> MESGIDLQGQFISALQSLGLSHDLAKLLWLPLPMLMMLIVATVGVLVAVWLERKISAAVQQRIGPEYIGPLGILAPLADGLKLIFKEDVLPANSDRWLFTLGPAVVVIPVFLSYIIVPFGQNLLISNLAMGVFLWIALSSIAPIGLLMAGYASNNKYSLLGGLRAAAQSISYEIPLALAVLAVAMMSNGLGTVEIVEQQSQYGILSWNVWRQPIGFLVFWIAALAECERLPFDLPEAEEELVAGYQTEYAGMKFALFYLGAYVNLVLSALLVSVLYFGGWSFPIPLETIANLLGVSETNPFLQIAFAVLGITMTLIKAYFFVFLAILLRWTVPRVRIDQLLDLGWKFLLPVGLVNLLLTAGLKLAFPVAFGG;> MDLVTLAGQLNAGTILPETILIVTLLVVLLADLIQGRQADRWTPYFAIVGLGGAIATMIPLWTQPATISFFGSFISDHLSLFFRGLIALSALGTILMSIRYVEQTGSSLGEFMTILLTATVGGMFIAGAQELVFIFVALETLSIASYLLTGYTKRDSRSNEAALKYLLIGAASSAIFLYGSSLLYGLSGGHTQLPAIAQALSSESLGLVVALVFVIAGISFKISAVPFHQWTPDVYEGAPTPVVAFLSVGSKAAGFALAIRFLTLAFPSVTDQWQLIFTVLAILSMILGNVVALAQTSMKRMLAYSSIGQAGFVMIGFVVGTEAGYASMLFYLLVYLFMNLGAFTCVILFSLRTGTDQISEYAGLYQKDPLLTLGLSLCLLSLGGIPPLAGFFGKIYLFWAGWQAGAYGLVLLGLLTSVISIYYYIRVVKMMVVKEPQEMSEAVRNYPEVSWSSFGLRPLQVGLVMTVIATSLAGILANPLFNLVNTAVWDVPQLANQPTVMEVAYQALSPAGKS;> MVAIPRLRDTATVFVLSGYEYFLGFLIICSLVPVLALAASALLRPKSGRMIRLTTYESGMEPIGGAWIQFNVRYYMFALVFVIFDVETVFLYPWAVAFHQLGLLAFIEALIFIAILVVALVYAWRKRALEWS;> MSTFPWLTTIILFPIVAALAIPFIPDPTGKGRPIRWYALAVGLIDFALIVYAFTNFYDLNTPGMQLWESYDWIPEIGLRWSVGADGLSMPLILLTGFITTLAILAAWPVTLKPRLFYFLMLAMYGGQIAVFAVQDMLVFFLAWELELIPVYLLLAIWGGHKRQYAATKFILYTAGSSLFILVAGLAMAFYGDTVSFDMQTLAAKDYALGFQLLVYAGFLVAYGVKLPIVPLHTWLPDAHGEATAPVHMLLAGILLKMGGYALIRMNVDMLPAAHAKFAPVLVILGVVNIIYAALTSYAQRNLKRKIAYSSISHIGFVLIGIASFTNLGMSGAVLQMVSHGLIGASLFFLVGATYDRTHTLILEEMGGVGQKMKKIFAMFTACSLASLALPGMSGFVAELMVFIGFATSDAYSLPFRVIVVFLAAVGVILTPIYLLSMLREIFYGPENKELVEHEALVDAEPREVFIIACLLVPIIGIGLYPKLLTQIYDATTGQVIARAREVLPTLAQQTEQPLGILPMVAPQLKANAQ;> MQLTYVLILAALLFCIGIYGLVTSRNAVRVLMSIELLLNAVNLNLIGFANYLDGQQIKGQVFAVFVITVAAAEAAVGLAIILAIYRNRDTVDMEKFNLLKW;> MEPLYQYAWLIPVLPLLGALIVGFGLIAFSETTSKLRRPSAIFIMALMAIAMGHSLTLFWSQVQGHLPYTQMIEWAAAGNLHIAMGYVIDPLAALMLVIVTTVAFLVMLYSDGYMAHDPGYVRFFAYLSLFGSSMLGLVVSPNLVQVYIFWELVGMCSYLLIGFWYDRKSAAEAAQKAFVTNRVGDFGLLLGMVGLFWATGTFDFAGMGDRLTELVNTGLLSPSLAAILAILVFLGPVAKSAQFPLHVWLPDAMEGPTPISALIHAATMVAAGVFLIARMFPVFEQLPQVMTTIAWTGAFTAFMGATIAITQNDIKKSLAYSTISQLGYMVMGMGVGAYSAGLFHLMTHAYFKAMLFLGSGSVIHSMEGVVGHNPDLAQDMRYMGGLRKYMPITGATFLVGCLAISGVPPFAGFWSKDEILGAVFHANPAMWLLTWLTAGLTAFYMFRMYFMTFEGKFRNVPPERQEHHDHHSHHAAVPHESPWTMTLPLVVLAIPSTLIGFVGTPFNNLFEVFIHAPGEEKVAEHAVDLTEFLILGGSSVGIGLMGITVAYLMYLKGTPSPQAIAKAIQPLYQFSLHKWYFDELYEAVFIKGCRRLARQVLEVDYNVVDGVVNLTGFVTMVTGEGLKYLQNGRAQFYALIVLLAVLGFVIFSVQT;> MDLATLTQTITFFALAAAVIIAALGVVLLDNVVYSAFLLGGVFLSIAGLYILMNADFVSAAQILIYVGAVNVLILFAIMLVNKRETYTPVPGRWLRQGGAAVVSLGVFALLTKMILQTPWQLSSVPPTPDSITTIGQHFFSDFLLPFELASVLLLMALIGAVVLARRELVLEPEPILGEEVVPPLELPERPREPVALSEK;> MPKIETRTEPMVINMGPHHPSMHGVLRLMVTLDGEDVIDCEPVIGYLHRGMEKIAENRTNIMFIPYVSRWDYAAGMFNEAVTVNAPEKLAGIPVPKRASYIRVIMLELNRIANHLLWLGPFLADVGAQTPFFYIFREREYIYDLFEAATGMRFINNNYFRIGGVAADLTYGWVTKCRDFCDYFLPKVDEYERLITNNPIFVRRLQGVGKISREEAINWGLSGPMLRASGVKWDLRKVDHYECYDDFDWDVPVATEGDCLARYIVRIQEMRESVKIIRQALDGLPGGPYENLEAKRMLEGAKSEWNGFDYQYIGKKLSPTFKIPKGEHYVRVESGKGELGIYLIGDDNVFPWRWKIRPPDFNNLQVLPQLLKGMKVADIVAILGSIDVIMGSVDR;> MKFLNQITNYAKEAVQSAKYIGQGLSVTFDHMRRRPITVQYPYEKLIPSERFRGRIHFEFDKCIACEVCVRVCPINLPVVDWVFNKELKKKELKHYSIDFGVCIFCANCVEYCPTNCLSVTEEYELATYDRHELNYDSVAMGRIPYKVTQDPMVTPIREFAYLPAGVMSGHDLPAGAQRAGERPEAIANTAKSSEN;> MSDTPEAPIVEAGPVGRLLQSQNLSVESLGRDASGVEMIKVDRDRLLAVCQTLYADGFNYLRCQAAYDSGPGQDLVSTYHLIKLSDNADRPPEVRIKVFVPRDDPRVPSVYWIWKTADWQERESYDMFGIVYEGHPNLKRILMPEDWVGWPLRKDYITPDFYELQEAY;> MTNTTSPAILNPIARPEVPQELAENIILTSLNDVYDWARLSSLWPLMYGTACCFIEFAAMIGSRFDFDRFGLVPRNSPRQADLIITSGTITMKMAPALVRLYEQMPSPKYVIAMGACTITGGMFSSDSYSAVRGVDKLIPVDVYLPGCPPRPEAIMDAIVKLRKKIANEHINERGNLAQTHRLFTAKHKMKPVPPILTGQYLNAPSRQAPPPALAAAMGIAVPALGEAVSETTSVAE;> MAVSTELLVLGVYGALAGLYLLVVPAIVYAYLNARWYVASSFERAFMYFLVTFFFPGLLLLAPFINFRPQPRSLNS;> MLLKSTTRHVHIYAGHVVDGEVHPDTETLTLNVDPDNELEWNEAALAKVEAKFRELVANAAGEDLTEYNLRRIGSDLEHFIRSLLMQGEIGYNLNSRVRNYSLGIPRVNHS;> MGLLAGYQFVKDLESAGALALFVPPEGGFEGRYQRRLRSKGYTTLPMSAPGLGDLAAYLTQEHGIRPAHTGKEDIRVYFQPPLVTYHLENLPPNAKGLVLWLIDGKRLSKQEFAYLAQLTQTLPKFKVVVEVGGDRVVRWEPLADWVAAA;> MAIKKGDLVKVVAEKLANSLEALASDHRYPPYLFEGRGEVVDIRGDYAQIKFPVPTPTVWLRLDQLEVAQ;> MDAVISVKPILLAMTPVFILLCLFFGTRNGFYDTDQYHGNGSAH;> MATDFNRGIMKFDGADSPAMIAISAVLILGFIAALIWWALHTAYA;> MIRPIADTYPLLPLSKAQMGQRQEIINSHKRLWDKTMATDLIMTILPGMTVKVTNPNDTYYQFQGIVQRITDGKVAVLFEGGNWDKLVTFQASE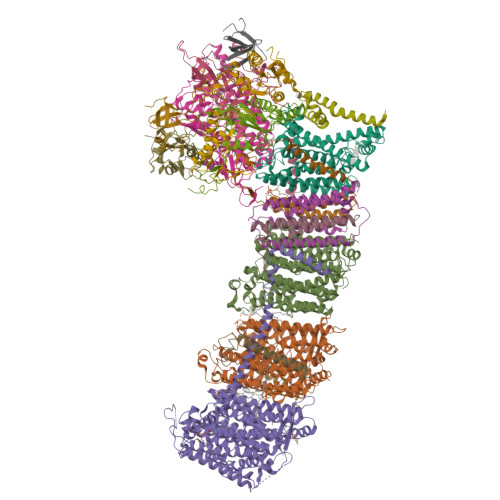LEPVVVTPKEKAKAKK6-(2-phenoxyphenyl)[1,2,4]triazolo[3,4-b][1,3,4]thiadiazole 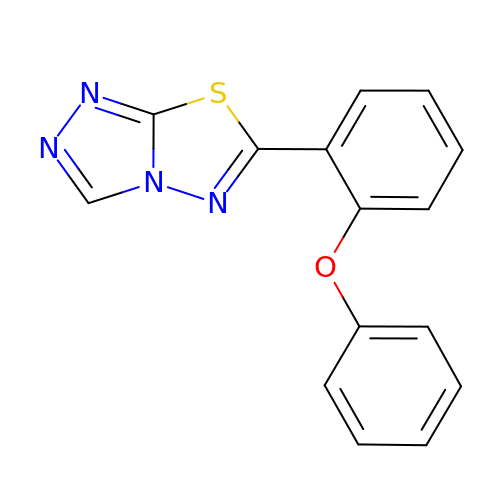| C15 H10 N4 O S | KCOSAQLZHSXLNP-UHFFFAOYSA-N> GPLGSGETVKIVRIEKARDIPLGATVRNEMDSVIISRIVKGGAAEKSGLLHEGDEVLEINGIEIRGKDVNEVFDLLSDMHGTLTFVLIPS;> RVEMWNLMPPPAMERLI

Apical localization of the Crumbs (Crb) transmembrane protein requires a PDZ-mediated interaction with Pals1 (protein-associated with Lin7, Stardust, MPP5), a member of the p55 family of membrane-associated guanylate kinases (MAGUKs). Pals1 belongs to the MPP family of proteins (membrane protein, palmitoylated), also known as the p55 subfamily of membrane-associated guanylate kinases (MAGUKs). Pals1 acts as a scaffold protein, recruiting other proteins to the apical domain of the cells: the L27 domains of Pals1 bind to Patj and Lin7, while the amino-terminal regions of Pals1 can interact with the PDZ domain of Par6, linking the Crb and Par complexes.

To define the molecular interaction between human Pals1PDZ and Crb17, we successfully crystallized the complex and determined its structure at 1.23 Å resolution. A single Pals1PDZ–Crb17 complex is present within the asymmetric unit. The Pals1PDZ adopts a canonical PDZ fold consisting of two β-sheets flanked by two α-helices. The total buried surface area between Pals1PDZ and Crb17 is ∼500 Å2. Leu321 of Pals1 adopts a strained side-chain rotamer on binding the ligand, allowing the side chain of Ile1406 from Crb17 to point into a deep hydrophobic pocket in Pals1PDZ. Van der Waals contacts between Crb17 Leu1405 and Pals1 Pro266 stabilize a closed carboxylate-binding loop enveloping the peptide ligand. Charged interactions with the ERLI motif are also found; Crb17 Glu1403 forms a salt bridge with Pals1PDZ Arg282 and also forms hydrogen bonds to the side chains of Thr270 and Ser281. In contrast, in the presence of the Crb17 peptide Phe318 swings out of the pocket to pack against the Arg1404 side chain of Crb17. Overall, the structure explains the tight conservation of each side chain of the Crb ERLI motif through selective interactions with the Pals1PDZ domain, consistent with the binding affinities measured in solution by fluorescence polarization. Our structure of a Crb17 peptide ligand bound to the Pals1 PDZ domain explains the basis for this conservation and presents detailed charged side-chain interactions, carboxylate-binding loop contacts and hydrophobic pockets for the penultimate two Crb residues.> PKHGKRYRALLEKVDPNKIYTIDEAAHLVKELAT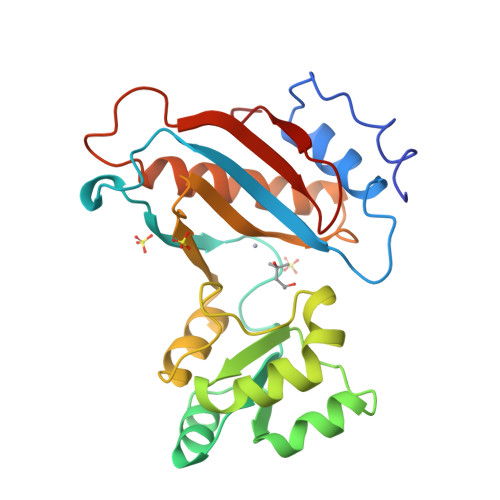AKFDETVEVHAKLGIDPRRSDQNVRGTVSLPHGLGKQVRVLAIAKGEKIKEAEEAGADYVGGEEIIQKILDGWMDFDAVVATPDVMGAVGSKLGRILGPRGLLPNPKAGTVGFNIGEIIREIKAGRIEFRNDKTGAIHAPVGKACFPPEKLADNIRAFIRALEAHKPEGAKGTFLRSVYVTTTMGPSVRINPHS(2E)-2-{2-[4-(3,4-dichlorophenyl)-1,3-thiazol-2-yl]hydrazinylidene}-3-(2-nitrophenyl)propanoic 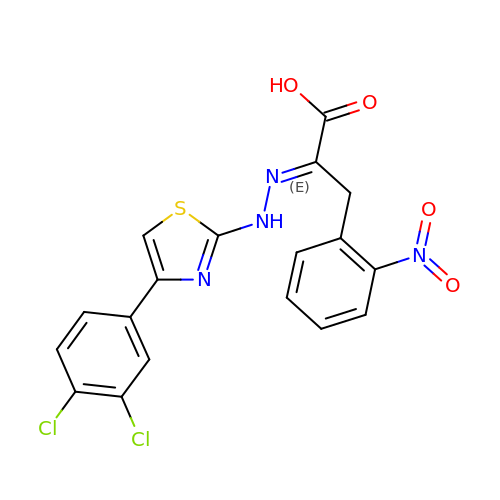acid | C18 H12 Cl2 N4 O4 S | KFRKRECSIYXARE-HYARGMPZSA-N5-(2-{[HYDROXY(PHOSPHONOOXY)PHOSPHORYL]OXY}ETHYL)-2-[(1Z)-1-HYDROXY-3-(PHOSPHONOOXY)PROP-1-EN-1-YL]-3-{[(4Z)-4-IMINO-2-METHYL-4,5-DIHYDROPYRIMIDIN-5-YL]METHYL}-4-METHYL-1,3-THIAZOL-3-IUM 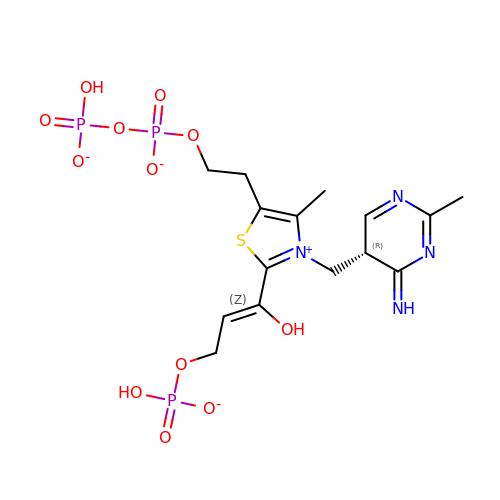| C15 H21 N4 O12 P3 S | IYJJFPCOWJABBY-AOCMNYQTSA-L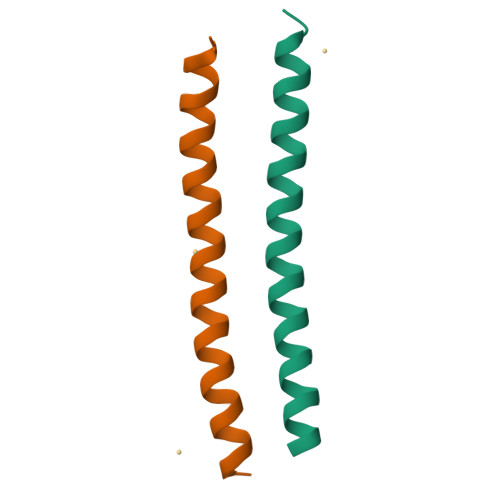>[2x]GSPELQNFLTILEKEEQDKIHQLQKKYNKFRQKLEEALRESQGKPG>PIVDTGSVAPLSAAEKTKIRSAWAPVYSTYETSGVDILVKFFTSTPAAQEFFPKFKGLTT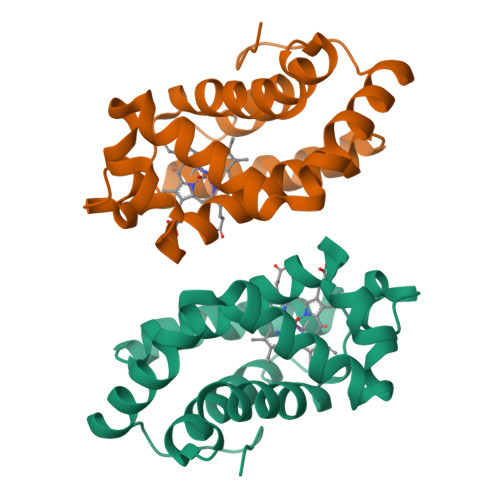ADQLKKSADVRWHAERIINAVNDAVASMDDTEKMSMKLRDLSGKHAKSFQVDPQYFKVLAAVIADTVAAGDAGFEKLMSMICILLRSAY[6x]METHYL 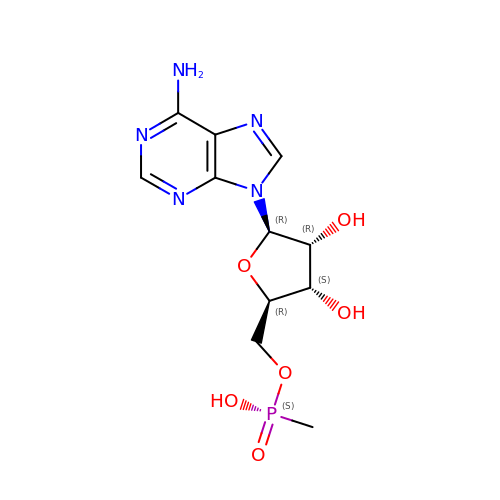PHOSPHONIC ACID ADENOSINE ESTER | C11 H16 N5 O6 P | PXSSQXBLDTZHLF-IOSLPCCCSA-N Examples include herpesviruses and most bacteriophages, both of which replicate their DNA as head-to-tail concatemers containing multiple copies of the genome that must be cleaved to generate unit-length viral genomes. This is achieved using a “terminase” complex, which, in bacteriophages comprises two proteins, termed Large (TerL) and Small (TerS) terminases; but in herpesviruses contains three separate components—pUL15, pUL28 and pUL33—in hitherto unknown oligomeric forms. The terminase complex recognizes a specific sequence or structure on the concatemeric DNA and cuts it to produce the free end where packaging is initiated. Acting as the packaging motor, the terminase complex then hydrolyzes ATP molecules to translocate negatively charged DNA into a space-limited procapsid through a dodecameric portal (Chen, 2020; Nan Wang, et al. 2020). Each subunit of the hexameric ring is a heterotrimer formed by three proteins (pUL15, pUL28 and pUL33) interdigitating with each other.

Here we reported the atomic structures of a herpesvirus hexameric terminase complex in both the apo and ADP•BeF3 bound states at 3.5 Å and 3.6 Å. To elucidate the structural mechanism of viral DNA packaging, we determined the cryoEM structures of the hexameric and dodecameric terminase assemblies in the apo state at 3.9 Å and 4.6 Å resolution, with C6 and D6 symmetry respectively; and those of the hexameric and dodecameric terminase bound with an ATP mimic, ADP•berylliumtrifluoride (ADP•BeF3, a nonhydrolyzable ATP analog to mimic ATP in physiological conditions) at 4.3 Å and 4.6 Å resolution, respectively. Herpesvirus terminases are known to be a member of the additional strand, conserved glutamate (ASCE) superfamily of ATPases however, our cryoEM structure of the herpesvirus hexameric terminase assembly shows that its size, with an external diameter of ~225 Å and a height of ~100 Å, is substantially larger than the dimensions of most ASCE members. The central channel of the hexameric ring, having a funnel-like shape with an internal diameter of 39 Å, can possibly bind and translocate the dsDNA substrate using specialized basic residues that project into the central channel. Expectedly, the central channel of the hexameric ring has a similar internal diameter to that of the dodecameric portal in herpesviruses, also suggesting the role in dsDNA translocation. In our structures, six copies of the ATPase domain are arrayed around the interior of the ring, forming a “funnel” like structure with a central channel. Remarkably, a large basic patch of six residues, R291, K292, R306, R313, K318 and R331, that are highly conserved in herpesviruses and bacteriophages, is observed lining the central channel, which is believed to bind DNA during translocation.

> TMGGDALRVPFLDFATATPKRHQTVVPGVGTLHDCCEHSPLFSAVARRLLFNSLVPAQLKGRDFGGDHTAKLEFLAPELVRAVARLRFKECAPADVVPQRNAYYSVLNTFQALHRSEAFRQLVHFVRDFAQLLKTSFRASSLTETTGPPKKRAKVDVATHGRTYGTLELFQKMILMHATYFLAAVLLGDHAEQVNTFLRLVFEIPLFSDAAVRHFRQRATVFLVPRRHGKTWFLVPLIALSLASFRGIKIGYTAHIRKATEPVFEEIDACLRGWFGSARVDHVKGETISFSFPDGSRSTIVFASSHNTNGIRGQDFNLLFVDEANFIRPDAVQTIMGFLNQANCKIIFVSSTNTGKASTSFLYNLRGAADELLNVVTYICDDHMPRVVTHTNATACSCYILNKPVFITMDGAVRRTADLFLADSFMQEIIGGQARETGDDRPVLTKSAGERFLLYRPSTTTNSGLMAPDLYVYVDPAFTANTRASGTGVAVVGRYRDDYIIFALEHFFLRALTGSAPADIARCVVHSLTQVLALHPGAFRGVRVAVEGNSSQDSAVAIATHVHTEMHRLLASEGADAGSGPELLFYHCEPPGSAVLYPFFLLNKQKTPAFEHFIKKFNSGGVMASQEIVSATVRLQTDPVEYLLEQLNNLTETVSPNTDVRTYSGKRNGASDDLMVAVIMAIYLAAQAGPPHT;> AAPVSEPTVARQKLLALLGQVQTYVFQIELLRRCDPHIGRGKLPQLKLNALQVRALRRRLRPGLEAQAGAFLTPLSVTLELLLEYAWREGERLLGSLETFATAGDVAAFFTETMGLARPCPYHQRVRLDTYGGTVHMELCFLHDVENFLKQLNYCHLITPSRGATAALERVREFMVGAVGSGLIVPPELSDPSHPCAVCFEELCVTANQGATIASRLADRICNHVTQQAQVRLDANELRRYLPHAAGLSDADRARALSVLDHALARTAGGDGQPHPSPENDSVRKEADALLEAHDVFQATTPGLYAISELQFWLASGDRAGQTTMDAFASNLTALARRELQQETAAVAVELALFGRRAEHFDRAFGSHLAALDMVDALIIGGQATSPDDQIEALIRACYDHHLTTPLLRRLVSPEQCDEEALRRVLARMGAGGAADAPKGGAGPDDDGDRVAVEEGARGLGAPGGGGEDEDRRRGPGGQGPETWGDIATQAAADVRERRRLYADRLTKRSLASLGRCVREQRGELEKMLRVSVHGEVLPATFAAVANGFAARARFCALTAGAGTVIDNRSAPGVFDAHRFMRASLLRHQVDPALLPSITHRFFELVNGPLFDHSTHSFAQPPNTALYYSVENVGLLPHLKEELARFIMGAGGSGADWAVSEFQRFYCFDGISGITPTQRAAWRYIRELIIATTLFASVYRCGELELRRPDCSRPTSEGRYRYPPGVYLTYDSDCPLVAIVESAPDGCIGPRSVVVYDRDVFSILYSVLQHLAPR;> TLRDTIPDCALRSQTLESLDARYVSRDGAHDAAVWFEDMTPAELEVVFPTTDAKLNYLSRTQRLASLLTYAGPIKAPDDAAAPQTPDTACVHGELLARKRERFAAVINRFLDLHQILR>MSYRMFDYLVPNVNFFGPNAISVVGERCQLLGGKKALLVTDKGLRAIKDGAVDKTLHYLREAGIEVAIFDGVEPNPKDTNVRDGLAVFRREQCDIIVTVGGGSPHDCGKGIGIAATHEGDLYQYAGIETLTNPLPPIVAVNTTAGTASEVTRHCVLTNTETKVKFVIVSWRNLPSVSINDPLLMIGKPAALTAATGMDALTHAVEAYISKDANPVTDAAAMQAIRLIARNLRQAVALGSNLQAREYMAYASLLAGMAFNNANLGYVHAMAHQLGG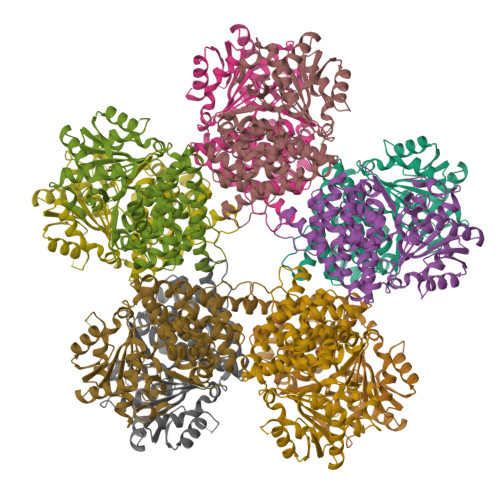LYDMPHGVANAVLLPHVARYNLIANPEKFADIAELMGENITGLSTLDAAEKAIAAITRLSMDIGIPQHLRDLGVKETDFPYMAEMALKDGNAFSNPRKGNEQEIAAIFRQAF[20x]>MRGETLKLKKDKRREAIRQQIDSNPFITDHELSDLFQVSIQTIRLDRTYLNIPELRKRIKLVAEKNYDQISSIEEQEFIGDLIQVNPNVKAQSILDITSDSVFHKTGIARGHVLFAQANSLCVALIKQPTVLTHESSIQFIEKVKLNDTVRAEARVVNQTAKHYYVEVKSYVKHTLVFKGNFKMFYDKRG[4x]

In order to shed light on this fundamental mechanism, we studied S. aureus FapR (SaFapR) a transcription factor that senses the levels of malonyl-CoA, a key intermediate in fatty acid biosynthesis, and modulates the expression of genes involved in fatty acid and phospholipid biosynthesis. FapR has been shown to globally repress the expression of the genes from the fap regulon encoding the soluble FASII system as well as two key enzymes that interface this pathway with the synthesis of phospholipid molecules. Like most transcriptional regulators in bacteria, FapR is a homodimeric repressor. Each protomer consists of a N-terminal DNA-binding domain (DBD) harboring a classical helix-turn-helix motif connected through a linker α-helix (αL) to a C-terminal effector-binding domain (EBD).

The structure of SaFapR in complex with the DNA operator revealed a strikingly different overall conformation of the protein, compared to those of the ligand-free and the effector-bound repressor. The crystal structure of SaFapR in complex with a 40-bp oligonucleotide comprising the PfapR promoter was determined at 3.15 Å resolution. Two SaFapR homodimers were observed to bind to a single DNA molecule in the crystal. Each protein homodimer exhibits an elongated asymmetric conformation in the crystal structure, in which the two DNA-bound DBDs are structurally detached from the central dimeric ‘hot-dog’ EBD. The amphipatic linker helix αL plays a major role in stabilizing the molecular architecture of the SaFapR-DNA complex. Helix αL interacts with αL′ from the second protomer mainly through its exposed hydrophobic face (including residues Ile59, Val62 and Ala63). The two DBDs from the asymmetric homodimer interact in a similar manner with DNA. The recognition helix α3 from the helix-turn-helix motif penetrates the double-helix major groove and makes extensive interactions with the two DNA chains. The SaFapR-DNA interface mainly involves the DNA backbone phosphates, except for base-specific interactions of Gln41 (from the recognition helix α3) in the major groove and Arg56 (from the linker helix αL) in the minor groove. Importantly, the insertion of the guanidinium groups of this arginine from both protomers promotes the opening of the minor groove, inducing a pronounced local bending of DNA.>MVDLEQEFALGGRCLAFHGPLMYEAKILKIWDPSSKMYTSIPNDKPGGSSQATKEIKPQKLGEDESIPEEIINGKCFFIHYQGWKSSWDEWVGYDRIRAYNEENIAMKKRLANEAKEAKKSLLE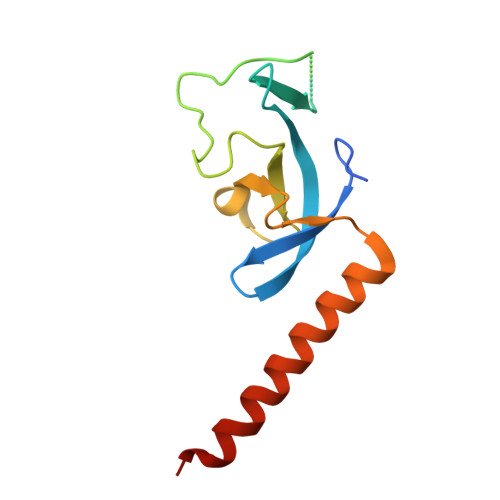HHHHHH[2x]>MHHHHHHENLYFQGMDGTVLKQLQPPPRGPRELEFYNMVYAADCFDGVLLELRKYLPKYYGIWSPPTAPNDLYLKLEDVTHKFNKPCIMDVKIGQKSYDPFASSEKIQQQVSKYPLMEEIGFLVLGMRVYHVHSDSYETENQHYGRSLTKETIKDGVSRFFHNGYCLRKDAVAASIQKIEKILQWFENQKQLNFYASSLLFVYEGSSQPTTTKLNDRTLAEKFLSGGGGSGGGGSQEIAEVEVRMIDFAHVFPSNTIDEGYVYGLK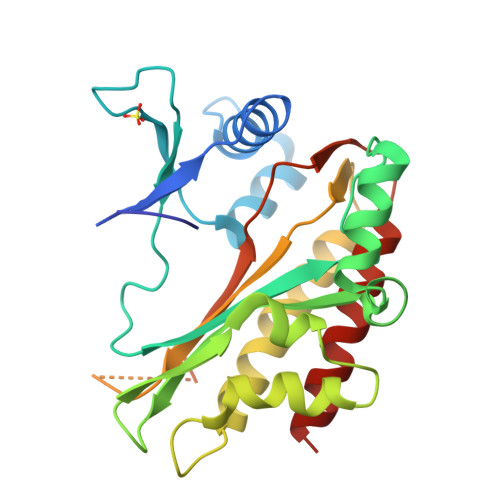HLISVLRSILDN[2x]> MFRQLKKNLVATLIAAMTIGQVAPAFADSADTLPDMGTSAGSTLSIGQEMQMGDYYVRQLRGSAPLINDPLLTQYINSLGMRLVSHANSVKTPFHFFLINNDEINAFAFFGGNVVLHSALFRYSDNESQLASVMAHEISHVTQRHLARAMEDQQRSAPLTWVGAL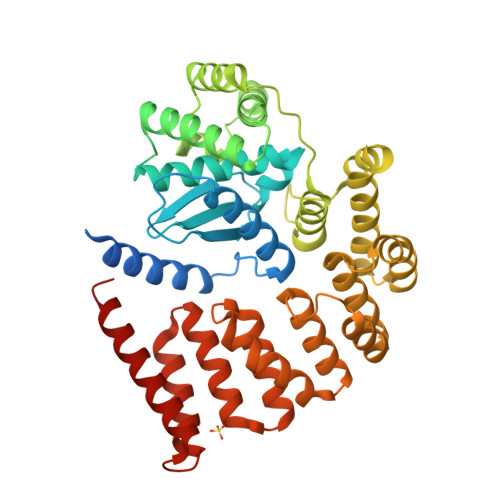GSILLAMASPQAGMAALTGTLAGTRQGMISFTQQNEQEADRIGIQVLQRSGFDPQAMPTFLEKLLDQARYSSRPPEILLTHPLPESRLADARNRANQMRPMVVQSSEDFYLAKARTLGMYNSGRNQLTSDLLDEWAKGNVRQQRAAQYGRALQAMEANKYDEARKTLQPLLAAEPGNAWYLDLATDIDLGQNKANEAINRLKNARDLRTNPVLQLNLANAYLQGGQPQEAANILNRYTFNNKDDSNGWDLLAQAEAALNNRDQELAARAEGYALAGRLDQAISLLSSASSQVKLGSLQQARYDARIDQLRQLQERFKPYTKM>[2x]MHHHHHHHHHHSGDEVDAGSGHMGTQKVTPALIFAITVATIGSFQFGYNTGVINAPEKIIKEFITKTLTDKGNAPPSEVLLTSLWSLSVAIFSVGGMIGSFSVGLFVNRFGRRNSMLIVNLLAVTGGCFMGLCKVAKSVEMLILGRLVIGLFCGLCTGFVPMYIGEISPTALRGAFGTLNQLGIVVGILVAQIFGLEFILGSEELWPLLLGFTILPAILQSAALPFCPESPRFLLINRKEEENAKQILQRLWGTQDVSQDIQEMKDESARMSQEKQVTVLELFRVSSYRQPIIISIVLQLSQQLSGINAVFYYSTGIFKDAGVQEPIYATIGAGVVNTIFTVVSLFLVERAG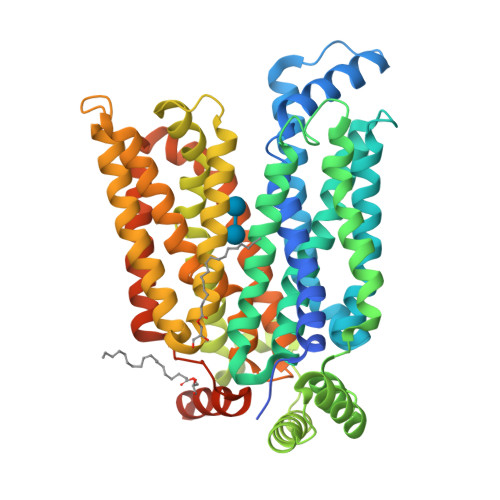RRTLHMIGLGGMAFCSTLMTVSLLLKDNYNGMSFVCIGAILVFVAFFEIGPGPIPWFIVAELFSQGPRPAAMAVAGCSNWTSNFLVGLLFPSAAHYLGAYVFIIFTGFLITFLAFTFFKVPETRGRTFEDITRAFEGQAHGADRSGKDGVMEMNSIEPAKETTTNV> SAMMYIQELRSGLRDMHLLSCLESLRVSLNNNPVSWVQTFGAEGLASLLDILKRLHDEKEETSGNYDSRNQHEIIRCLKAFMNNKFGIKTMLETEEGILLLVRAMDPAVPNMMIDAAKLLSALCILPQPEDMNERVLEAMTERAEMDEVERFQPLLDGLKSGTSIALKVGCLQLINALITPAEELDFRVHIRSELMRLGLHQVLQELREIENEDMK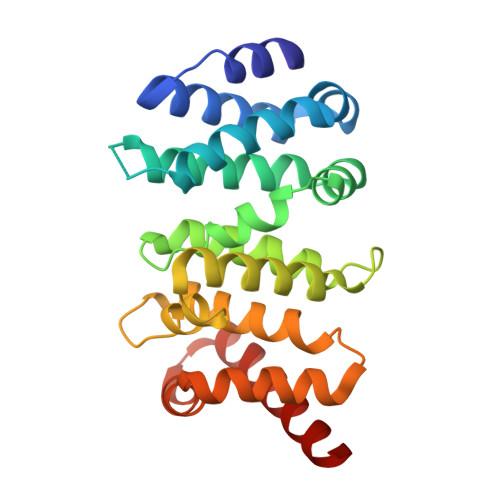VQLCVFDEQGDEDFFDL N-(2-acetamidoethyl)-2-nitro-ethanamide | C6 H11 N3 O4 | 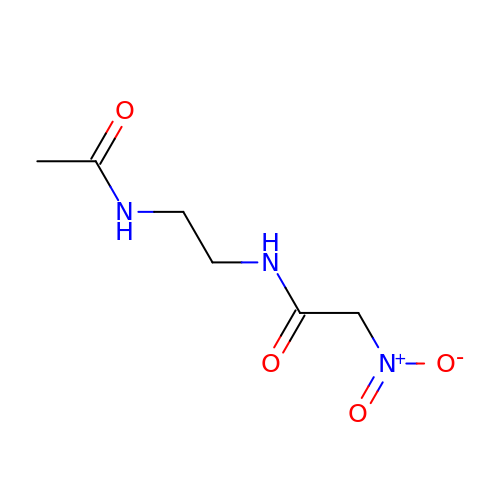XUBGUOZSRHKRMS-UHFFFAOYSA-N>[2x]MSQEVIRGIALPPAAQPGDPLARVDTPSLVLDLPAFEANLRAMQAWADRHEVALRPHAKAHKCPEIALRQLALGARGICCQKVSEALPFVAAGIRDIHISNEVVGPAKLALLGQLARAAKISVCVDNAENLAQLSAAMTRAGAEIDVLVEVDVGQGRCGVSDDATVLALAQQARALPGLNFAGLQAYHGSVQHYRTREERAAVCRQAARIAASYAQLLRESGIACDTITGGGTGSVEFDAASGVYTELQAGSYAFMDSDYGANEWNGPLKFQNSLFVLSTVMSTPAPGRVILDAGLKSTTAECGPPAVYGEPGLTYAAINDEHGVVRVEPGAQAPALGAVLRLVPSHVDPTFNLHDGLVVVKDGVVQDVWEIAARGFSR

Threonine aldolases are pyridoxal phosphate (PLP) dependent enzymes which catalyze the reversible cleavage of β-hydroxy amino acids (e.g. threonine) into glycine and the corresponding aldehyde (e.g. acetaldehyde). Thus, they can be classified into D-threonine aldolases (DTAs, EC 4.1.2.42) and L-threonine aldolases (LTAs, EC 4.1.2.5). First D-threonine aldolase encoding genes were discovered in 1997 and Liu et al. showed that DTAs are PLP-dependent and additionally need divalent ions to be catalytically active. Based on homology models, these enzymes were classified as belonging to the alanine racemase family (fold-type III) indicating a different evolutionary origin compared to LTAs.

Here, we report on the determination of the crystal structure of the DTA from Alcaligenes xylosoxidans (AxDTA) at 1.5 Å resolution. The crystal contained two molecules per asymmetric unit connected by a non-crystallographic two-fold axis. Each protomer comprises an alanine-racemase-like domain with an eight-stranded α/β-barrel (residues 32–274) together with a β-strand domain consisting of residues from the N-terminus (residues 1–31) and the C-terminus (residue 275–379). The structure of the AxDTA dimer is similar to dimers of alanine racemases and involves non-covalent contacts between both subdomains in a head-to-tail arrangement. Clear, residual electron density in the active site of both protomers was modeled by a molecule of pyridoxal phosphate (PLP) in two alternate conformations: covalently linked to Lys59 (occupancy ~40%) and non-covalently bound (occupancy ~60%). In both cases, the pyridine ring of PLP forms π-stacking interactions with Tyr187 (distance ~3.7 Å). The ion is coordinated only by two amino acid residues, His347 (via the Nε atom, 2.2 Å) and Asp349 (via the carboxylate, 2.2 Å), both from the alanine-racemase-like domain. Four water molecules (distances from 1.8 to 2.3 Å) complete a distorted octahedral coordination sphere. The metal binding site is located at approximately 5 Å distance from the aldehyde group of PLP and the manganese ion is nearly coplanar with the pyridine ring (0.4 Å out of the plane). The role of the essential metal (manganese) ion is most likely to activate the β-hydroxy group of the substrate for deprotonation by His193.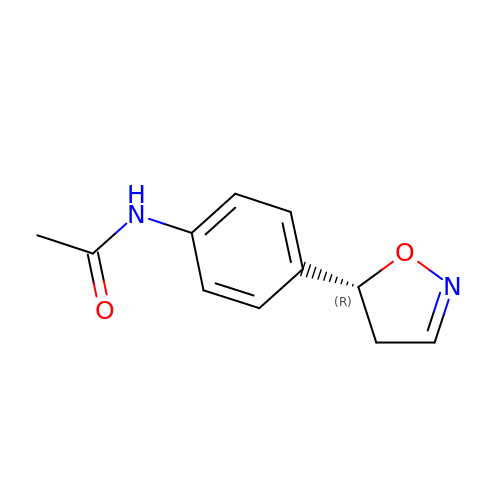~{N}-[4-[(5~{R})-4,5-dihydro-1,2-oxazol-5-yl]phenyl]ethanamide | C11 H12 N2 O2 | NXJZQAOQHFVDJW-LLVKDONJSA-N> RAITVFSPDGRLFQVEYAREAVKKGSTALGMKFANGVLLISDKKVRSRLIEQNSIEKIQLIDDYVAAVTSGLVADARVLVDFARISAQQEKVTYGSLVNIENLVKRVADQMQQYTQYGGVRPYGVSLIFAGID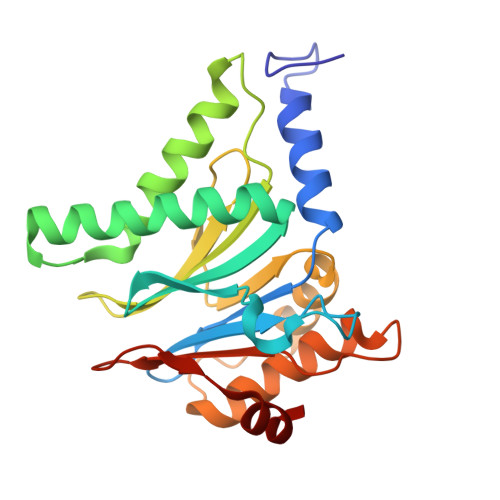QIGPRLFDCDPAGTINEYKATAIGSGKDAVVSFLEREYKENLPEKEAVTLGIKALKSSLEEGEELKAPEIASITVGNKYRIYDQEEVKKFL>SNAMKIGIIGVGKMASAIIKGLKQTPHELIISGSSLERSKEIAEQLALPYAMSHQDLIDQVDLVILGIKPQLFETVLKPLHFKQPIISMAAGISLQRLATFVGQDLPLLRIMPNMNAQILQSSTALTGNALVSQELQARVRDLTDSFGSTFDISEKDFDTFTALAGSSPAYIYLFIEALAKAGVKNGIPKAKALE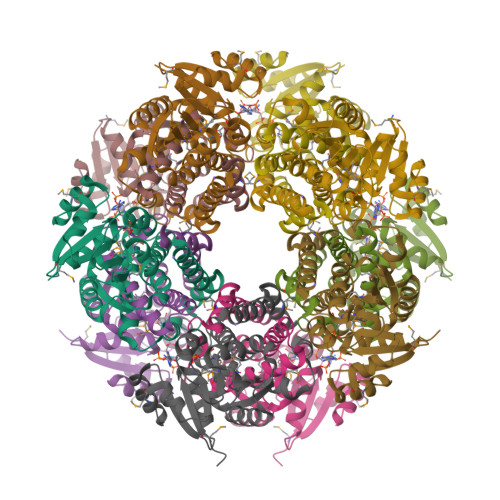IVTQTVLASASNLKTSSQSPHDFIDAICSPGGTTIAGLMELERLGLTATVSSAIDKTIDKAKSL[5x]> GHMKLRYIINENKLVFTSCNMRDKIITGKKIIFSQSVAKDQTKNLSSFLSERFYSVNQSHNHSIIIGSSLSHQENDIEHDTILDTSGVLVTTDTNGIVNGARVAITDGLGGGNGDQEEDDEIYRVSHSSCENFLNCDQNIDTTLSLITQPKASDKKQTAPKTLQHTEASMAAFIYQNHPGKGYIGEFANIGDGLIIILDKRFKIKHMVSACHIYRGFGTWTPPSLQALATTANKDALLVRQTLKLAEGDIIISMTDGVWGELKTSLIAQTNDRRDIGVDKEYFKTLFDELTDAPYPSSFDIARIITQRAMSRSLERRKTLIKLINEIEQQHFHEKSVKTINEVLEYFIKTGHVETAQTLKAILFEDGLSDGITYFENIEIPLEMVMHDLKSRTVGDCSTINVTRIPYHLDELIRGFINYPEKHQILAPLFKARVKSEADLEEAFHRLSLEMVQPEIECPISETHFERAFKKETLDKTQAVLTHYFRISTGLDSKKNYQERLNDLSAYLSKESSLEKNDIKLLLSMLDSEIKPKTGVFQTLFGENQNKLYKAFHKKIELQLLDSEIENKNELK

Legionella pneumophila, the causative agent of Legionnaires disease, secretes the enzyme AnkX that uses cytidine diphosphate-choline to post-translationally modify the human small G-Protein Rab1 with a phosphocholine moiety at Ser76. Later in the infection, the Legionella enzyme Lem3 acts as a dephosphocholinase, hydrolytically removing the phosphocholine. Through crystal structures of Lem3 in the apo form and in complex with Rab1b, we reveal Lem3’s catalytic mechanism, showing that it acts on Rab1 by locally unfolding it. Since Lem3 shares high structural similarity with metal-dependent protein phosphatases, our Lem3:Rab1b complex structure also sheds light on how these phosphatases recognise protein substrates.

In order to obtain structural insights into Lem3, we crystallised the full-length protein comprising the amino acids (aa) 1-570 (Lem3FL) and a shortened construct (aa 21-486, Lem321-486). We solved the structures of Lem3FL and Lem321-486 at 3.6 Å and 2.2 Å resolution, respectively. A superimposition of the Lem321-486 crystal and the AF2-predicted structure revealed high similarity (0.88 Å RMSD (root-mean-square deviation) on 444 superimposed Cα-atoms). Furthermore, we were able to solve the structure of Lem3FL by molecular replacement using the short construct structure and further extend the building of the C-terminal part with help of the AF2 model of Lem3FL. Lem3FL extends the fist opposite from the thumb by three α-helices (α18-α20, aa 495-567). Together with α-helices α14-α17, these three helices form a helical bundle consisting of helices α14-α20. In addition to the catalytic domain, we also provide a structure of the C-terminal part of Lem3, consisting of seven helices forming a bundle. Many PPM like-shaped proteins possess such C-terminal bundles, including SidD. A hydrophobic loop within the C-terminal helical bundle of SidD was shown to be responsible for membrane-localisation at the Golgi apparatus. Since SidD also targets Rab1 during the infection we speculate that the C-terminal part of Lem3 might have a similar function and is responsible for Lem3-localization close to its target protein. However, a corresponding hydrophobic loop could not be identified in Lem3.> NLRSLLVNPEGPTLMRLNSVQSSERPLFLVHPIEGSTTVFHSLASRLSIPTYGLQCTRAAPLDSIHSLAAYYIDCIRQVQPEGPYRVAGYSYGACVAFEMCSQLQAQQSPAPTHNSLFLFDGSPTYVLAYTGSYRAKLTPGCEAEAETEAICFFVQQFTDMEHNRVLEALLPLKGLEERVAAAVDLIIKSHQGLDRQELSFAARSFYYKLRAAEQYTPKAKYHGNVMLLRAKTGGAYGEAAGADYNLSQVCDGKVSVHVIEGDHATLLEGSG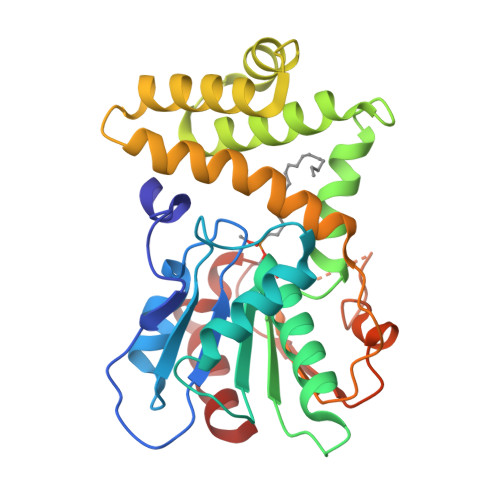LESIISIIHSS>AVSLDRTRAVFDGSEKSMTLDISNDNKQLPYLAQAWIENENQEKIITGPVIATPPVQRLEPGAKSMVRLSTTPDISKLPQDRESLFYFNLREIPPRSEKANVLQIALQTKIKLFYRPAAIKTRPNEVWQDQLILNKVSGGYRIENPTPYYVTVIGLGGSEKQAEEGEFETVMLSPRSEQTVKSANYNTPYLSYINDYGGRPVLSFICNGSRCSVKKEK[4x];>[4x]APTIPQGQGKVTFNNTVVDAPCSISQKSADQSIDFGQLSKSFLEAGGVSKPMDLDIELVNCDITAFKGGNGAKKGTVKLAFTGPIVNGHSDELDTNGGTGTAIVVQ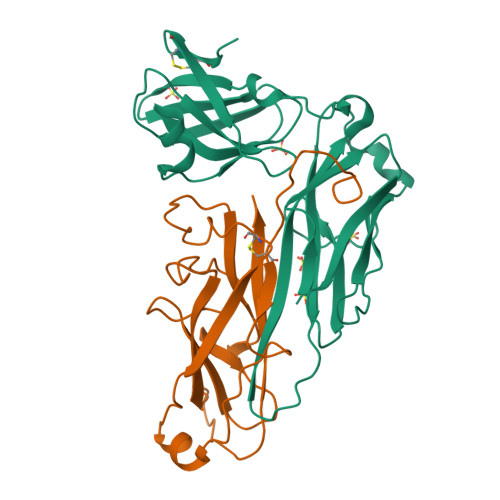GAGKNVVFDGSEGDANTLKDGENVLHYTAVVKKSSAVGAAVTEGAFSAVANFNLTYQ>MTFTILPAVDVVNGQAVRLDQGEAGTEKSYGTPLESALRWQEQGAEWLHFVDLDAAFNRGSNHELMAEITRQLDIKVELTGGIRDDASLERALATGATRVNIGTAALEKPEWIADVIRRHGEKIAVDIAVRLENGEWRTKGNGWVSDGGDLWEVLERLDSQGCSRFVVTDVSKDGTLTGPNVDLLRDVAAATDAPIVASGGISTLEDVLGLAKYQDEGIDSVIIGKALYEHRFT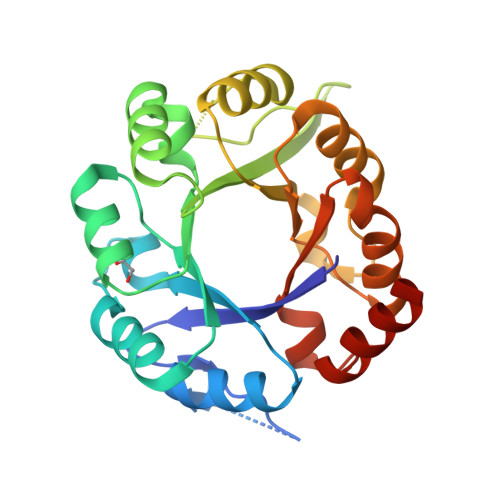LAEALEAVEKLGKLAA[2x]> DPSEYCSHMIGSGHLQSLQRLIDSQMETSCQITFEFVDQEQLKDPVCYLKKAFLLVQDIMEDTMRFRDNTPNAIAIVQLQELSLRLKSCFTKDYEEHDKACVRTFYETPLQLLEKVKNVFNETKNLLDKDWNIF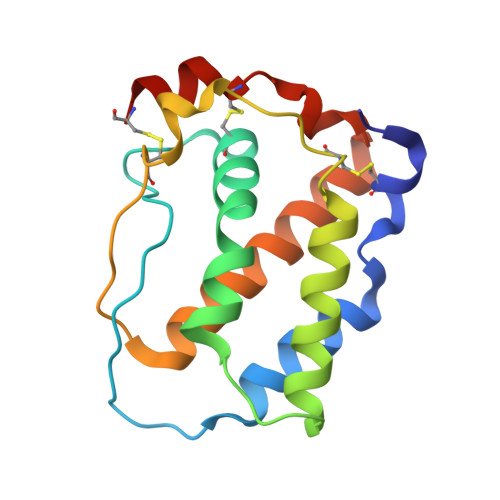SKNCNNSFAECSS Mfsd2a is the transporter for docosahexaenoic acid (DHA), an omega-3 fatty acid, across the blood brain barrier (BBB). Mechanistic studies revealed that Mfsd2a is a symporter for Na+ and is selective towards long chain, unsaturated fatty acids including DHA (22:6), α-linolenic acids (ALA, 18:3), and oleic acids (18:1) that are covalently tethered to the zwitterionic lysophosphatidylcholine (LPC) headgroup. Like other MFS members, drMfsd2a is comprised of twelve TMs that pack against one another with the substrate binding channel located at a cleft between the N- and C-terminal domains. Here, we present five structures of the Zebrafish (Danio rerio) isoform B Mfsd2a (drMfsd2a) in the inward-facing conformation determined by single-particle cryo-electron microscopy (cryo-EM), in the ligand-free state and displaying lipid-like densities at four distinct positions modeled as ALA-LPC.

We expressed and purified drMfsd2a from SF-9 insect cells and discovered that the protein copurified with endogenous phospholipids. We therefore modeled ALA-LPC into the four distinct lipid-like densities termed Lysolipid1A, 1B, 2B, 3C (numbers and letters refer to the lipid and LPC binding positions). Initial data processing yielded a 2.9 Å resolution map with three lipid-like densities representing three merged ligands, Lysolipid1A, 2B, 3C. However, our in vitro analysis indicates that there is only ~1 phospholipid per protein molecule, suggesting that the lipids observed in this model is a merge of particles of substrates bound at three separate sites. To gain more accurate assessment of how drMfsd2a coordinates these ligands, we plotted the intermolecular Lysolipid2C- and Lysolipid3C-drMfsd2a interactions using the model for the merged ligand map at 2.9 Å resolution. In drMfsd2a, the four lysolipids are positioned along the vertical axis of the substrate tunnel within a cleft between the N- and C-domains comprise of helices 1, 2, 4, 5, 7, 8, 9, 10, and 11 that open to the cytoplasmic side. Since Mfsd2a transports lipid-LPC from the outer to the inner leaflet, we propose the following order for the four ALA-LPC during substrate transport through Mfsd2a: Lysolipid1A, Lysolipid1B, Lysolipid2B, then Lysolipid3C.

> MHHHHHHHHHHENLYFQGGSDEVKLAKHETKSRLSVCSKLCYAIGGAPYQITGCAIGFFLQIYLLDVALLDPFYASIILFVGRAWDAVTDPTVGFLVSRTPWTRFGRMMPWIVLSTPFAVLCYFLIWYVPSVDQGKVVWYLIFYCCFQTLQTCFHVPYSALTMFISTEQKERDSATAYRMTVEVLGTLIGTAIQGQIVGMANAPCISTEIDLQSTGLEVAPDVQITDPHVSLQDLRNAYMIASGVICAIYVVCAVVLFLGVKEQKDTCRVRTEPMSFFQGICMVMGHGPYAKLVMGFLFTSLAFMLLEGNFALFCIYNLGFRNDFQNVLLVIMLSATLAIPFWQWFLTKFGKKTAVYIGTTSVVPFLISVVLVPSSLAVTYIASFAAGVSVAAAFLLPWSMLPDVVDDFKVQNPESQGHEAIFYSFYVFFTKFASGVSLGVSTLSLDFAGYVTRGCTQPGEVKLTLKILVSAAPIVLIIIGLLIFISYPINEEKRQGNRKLLNEQREQ;> ALDINSPEAEKNAKGARARITCNAGNQVGSAVAWFNQRPGDPASLLTYWAATEKGVAGKQSAQGASTKFSMSSAGPEAPSLSSYWCLLFEKGAFSFGGSKLNPREGAGPQASILPPSADLNTSGGAAVVCFLPNWYGNITVQWKTEAPQSQANMSWPGQAGANAAYAMAAVLAITKGDYGPGSFTCNASNRGTGPFAMSLN;> ASKLELSGPAEPRGSKSAQITCKAKGFPEARFWVFWLFQRAAALDWPAANFSGGPVQFESRFQGNASLKGSQAQANAELNIGALGSSTATYRCGWKLANGGFFPSWGGANVNGAAGAKAPAVYPVEISGAGTGSVTLGCLVKGYNAKPNLTWPGASGALTFPSELNGALWNLASAVTGSGFPSATCAVGFGAATDVDKKVAAA>SKNKEDKRNAEYRLAFEQLNFVGADSKTPILKSFIEDKGTRIDEITFESMIPIETWKSYIPQLQTSLNISIISIEQGASKRIVIIKSMAGDAKIPKYLPWDDKYIEEQEGVVVVGQTFSGNIKIDLNKSPHILSAGETGSGKSVILRCILWQLLKQGAIAYMVDFKGGVEFGLEYEKVGQVITEVDAAEKLFKYLVDENAKRLKLLRESGSKNIGEYNKKFEGEELKRIIVVIDELAELMDKTGVDDETRAKLVRIEGYTSTLARLSRATGINLCIGVQRPDAKVITGQIKNNV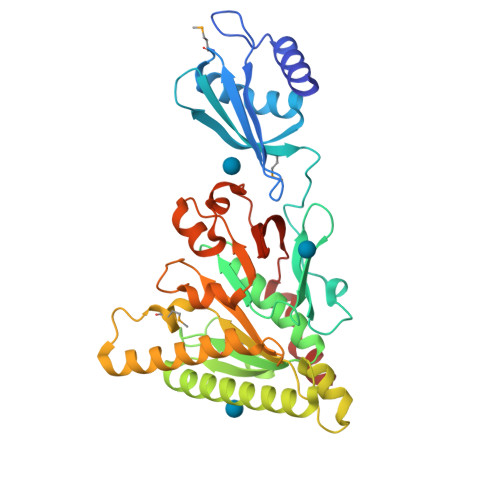PVRICGRFADSKASEIVLSNTKAKDLPEVKGRFLFKLGADTVQFQAFYFDDDKHFIPNKILKLR[2x]>[5x]GFQKIPVALLTTTGRKTGQPRVNPLYFLRDGGRVIVAASKGGAEKN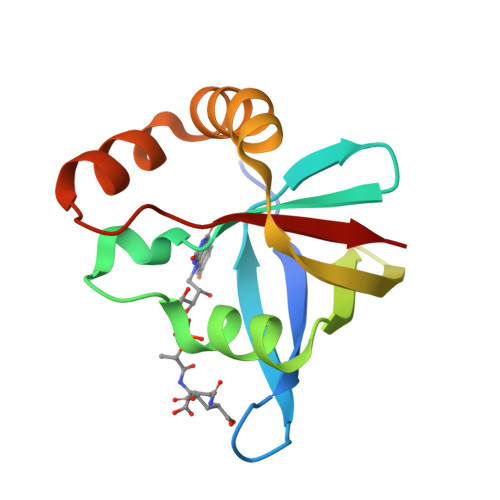PMWYLNLKANPKVQVQIKKEVLDLTARDATDEERAEYWPQLVTMYPSYQDYQSWTDRTIPIVVCEP>MATFVRNAWYVAALPEELSEKPLGRTILDTPLALYRQPDGVVAALLDICPHRFAPLSDGILVNGHLQCPYHGLEFDGGGQCVH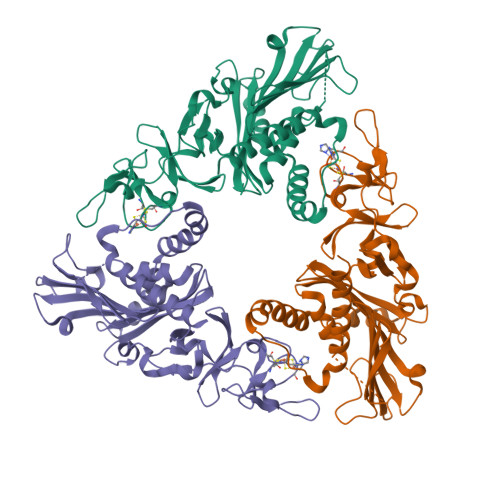NPHGNGARPASLNVRSFPVVERDALIWIWPGDPALADPGAIPDFGCRVDPAYRTVGGYGHVDCNYKLLVDNLMDLGHAQYVHRANAQTDAFDRLEREVIVGDGEIQALMKIPGGTPSVLMAKFLRGANTPVDAWNDIRWNKVSAMLNFIAVAPEGTPKEQSIHSRGTHILTPETEASCHYFFGSSRNFGIDDPEMDGVLRSWQAQALVKEDKVVVEAIERRRAYVEANGIRPAMLSCDEAAVRVSREIEKLEQLEAARLEHHHHHH[3x]>[2x]MNRKWEAKLKQIEERASHYERKPLSSVYRPRLSKPEEPPSIWRLFHRQAQAFNFVKSCKEDVHVFALECKVGDGQRIYLVTTYAEFWFYYKSRKNLLHCYEVIPENAVCKLYFDLEFNKPANPGADGKKMVALLIEYVCKALQELYGVNCSAEDVLNLDSSTDEKFSRHLIFQLHDVAFKDNIHVGNFLRKILQPALDLLGSEDDDSAPETTGHGFPHFSEAPARQGFSFNKMFTEKATEESWTSNSKKLERLGSAEQSSPDLSFLVVKNNMGEKHLFVDLGVYTRNRNFRLYKSSKIGKRVALEVTEDNKFFPIQSKDVSDEYQYFLSSLVSNVRFSDTLRILTCEPSQNKQK

PrimPol is a human DNA polymerase-primase that localizes to mitochondria and nucleus and bypasses the major oxidative lesion 7,8-dihydro-8-oxoguanine (oxoG) via translesion synthesis, in mostly error-free manner. PrimPol is important for both nuclear and mtDNA replication and belongs to the archaeo-eukaryotic primase-polymerase family that differs from other DNA polymerases by possessing a primase activity. The PrimPol catalytic core clasps the template-primer by two α/β modules, ModN and ModC. ModN (residues 35−105) interacts primarily with the template DNA strand and the template oxoG base, whereas ModC (residues 108−200 and 261−348) carries the catalytic residues Asp114, Asp116, and Glu280 and interacts with the incoming dCTP nucleotide: functions normally associated with the finger and palm domains of DNA polymerases, respectively.

The 2.1 Å resolution structure of PrimPol, extending a correct primer C opposite the oxoG, depicts the next step in accurate bypass of this oxidative lesion. The structure of the extension complex is almost identical to the unmodified complex (rmsd of ~0.46 Å over 249 Cαs of molecule A, for example). To capture the extension step we used a 17 nt DNA template (5′-CAT(oxoG)CCTACCACACCCC–3′), where the oxoG lesion is moved one base downstream compared to its location in the insertion complex, and 13 nt DNA primers with either a C or an A 2′-deoxy-3′-terminal bases (5′-GGGTGTGGTAGGX-3′, where X is C or A), and the next correct incoming base dATP. Thus, the T3 template base, which is 5′-adjacent to the oxoG residue, is now paired with the incoming dATP. The oxoG(anti) at the extension position of the active site is in a Watson−Crick base pair configuration with the 2′-deoxy-3′-C14 terminal primer base. Surprisingly, the conformation of the phosphate group of the oxoG is similar to that of the phosphate of an unmodified residue at the same position of the PrimPol complex (the C template strand residue in the undamaged complex). The steric clash of the O8 atom with the sugar-phosphate backbone that arises with oxoG(anti) is alleviated by adjustments of the backbone torsion angles of the phosphate group and a slight rotation of the sugar ring compared to the values observed for B-DNA. Thus, the conformation of the sugar-phosphate backbone of the template base at the extension position of the PrimPol active site is preset to accommodate the oxoG(anti). Overall, the oxoG(anti) template strand residue is accommodated at the extension position without significant adjustments to the active site or to the position of its partner primer terminal C residue, compared to the unmodified structure. This correlates with the near-normal efficiency extension from oxoG•C pair by PrimPol (∼75−85% of that observed for undamaged DNA).>MAMKAYSMLNVTATLDGRRVIGLMDGDDAITTSPGVDVGTMLVGADGSWLFSQTADKSATVVIKLKPNSPTHRQLTEKWMAQRAGRLVGFPFDFIDSASNEGGTGAEFFIQKAPDDSKGNNAVVREWTIVTGEWTPTIPTLL[18x];>[12x]MAKLPYSRVTNVTLTRTDNFPTRRGFGTQLILTHTAVSGQVDATKRTKLYASLAEVEADYPANTSVYKAALSAFSQNPRPIRL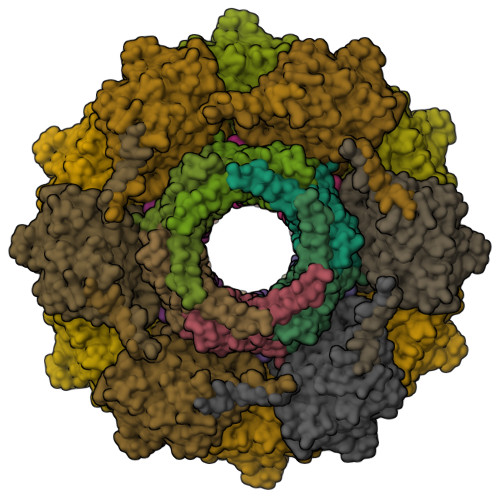KVGYAATPTGGDDAAKKADFITSLGAILNYDQAFYQITLDAALRDQPYLDGLVEWVEAQPKIAMIDSNAAGHEDPANTTVIAARHKGTVERTAVFYHTDSTEYLAASMAAYMSTRVFDDANSAYTLKFKKAPGVRAIDKGSAVVTAITGFVEQTGQSESAGHCANTLIDIGDQEFLVEGSTLTQNVFLDEIHATDWIIARTEEEMLSLFLNNDRVPFTDQGMQQLASVPRAIMQLAARAGIVALDLNPLTGAYEPAYTITVPSVFDIPESQRKARIAPAIQVRFRYAGAVHYSVINYTMTF N-({2-[2-chloro-4-(methoxymethoxy)phenyl]-1,3-thiazol-4-yl}acetyl)glycine | C15 H15 Cl N2 O5 S | 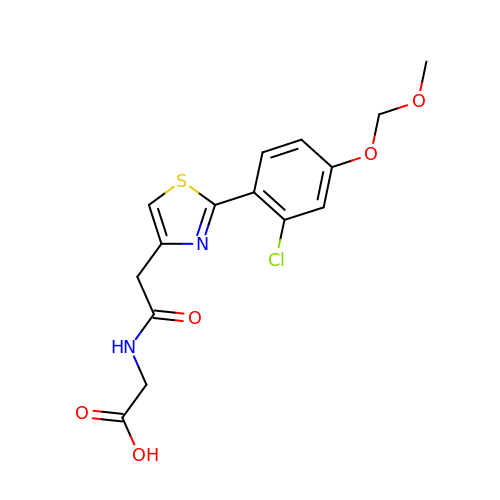MOVMDJVZNRFJJJ-UHFFFAOYSA-N>GSSGSSGMQIGKIIKVSGPLVMAENMSEACIQDMCLVGDLGVIGEIIEMRQDVASIQVYEETSGIGPGEPVRSTGEALSVELGPGIISQMFDGIQRPLDTFMEVTQSNFLGRGVQLPALDHE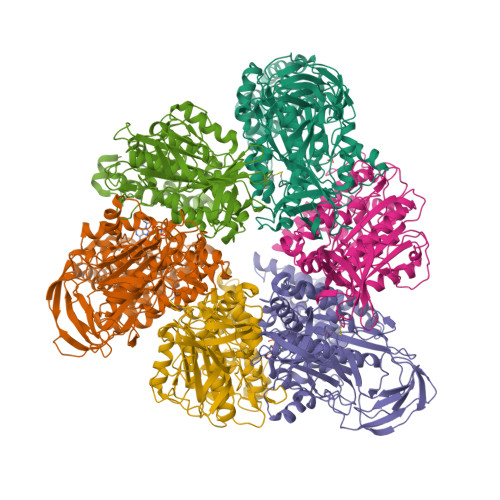KQWWFEATIEEGTEVSAGDIIGYVDETKIIQHKIMVPNGIKGTVQKIESGSFTIDDPICVIETEQGLKELTMMQKWPVRRGRPIKQKLNPDVPMITGQRVIDTFFPVTKGGAAAVPGPFGAGKTVVQHQIAKWSDVDLVVYVGCGERGNEMTDVVNEFPELIDPNTGESLMERTVLIANTSNMPVAAREASIYTGITIAEYFRDMGYDVAIMADSTSRWAEALREMSGRLEEMPGDEGYPAYLGSRLAEYYERSGRVIALGSDQREGSITAISAVSPSGGDISEPVTQNTLRVVKVFWGLDSSLAQKRHFPSINWIQSYSLYSTEVGRYMDQILQQDWSDMVTEGMRILQEEEQLNEIVRLVGIDSLSDNDRLTLEVAKSIREDYLQQNAFDDVDTFTSREKQFNMLKVILTFGKEARKALSLGAYFNEIMEGTVAVRERISRSKYIPEEELAKISSINEEIKETIQLIVSEGGMTDD[6x];>GSSGSSGMIKEYRTIKEVVGPLMAVEKVSGVKYEELIEVRMQNGEIRRGQVLEVQEDKAMVQIFEGTSGICLKNSSVRFLGHPLQLGVSEDMIGRVFDGLGRPKDNGPEILPEKYLDINGEVINPIARDYPDEFIQTGISAIDHLNTLVRGQKLPVFSGSGLPHKELAAQIARQATVLDSSDDFAVVFAAIGITFEEAEFFMEDFRQTGAIDRSVMFMNLANDPAIERIATPRMALTAAEYLAYEKGMHVLVIMTDMTNYAEALREISAARREVPGRRGYPGYLYTNLATLFERAGRIRGLKGSVTQIPILTMPEDDKTHPIPDLTGYITEGQIILTRELYKSGIQPPIDVLPSLSRLKDKGTGAGKTREDHAATMNQLFAAYAQGKQAKELAVVLGESALSDIDKIYAKFAERFENEYVNQGFYTNRTITETLDLGWELLAMLPRTELKRIKDDLLDKYLPEGK[6x]>MDSQRNLLVIALLFVSFMIWQAWEQDKNPQPQAQQTTQTTTTAAGSAADQGVPASGQGKLISVKTDVLDLTINTRGGDVEQALLPAYPKELNSTQPFQLLETSPQFIYQAQSGLTGRDGPDNPANGPRPLYNVEKDAYVLAEGQNELQVPMTYTDAAGNTFTKTFVLKRGDYAVNVNYNVQNAGEKPLEISTFGQLKQSITLPPHLDTGSSNFALHTFRGAAYSTPDEKYEKYKFDTIADNENLNISSKGGWVAMLQQYFATAWIPHNDGTNNFYTANLGNGIAAIGYKSQPVLVQPGQTGAMNSTLWVGPEIQDKMAAVAPHLDLTVDYGWLWFISQPLFKLLKWIHSFV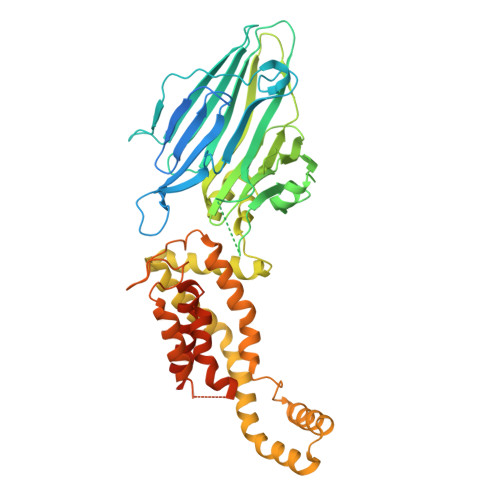GNWGFSIIIITFIVRGIMYPLTKAQYTSMAKMRMLQPKIQAMRERLGDDKQRISQEMMALYKAEKVNPLGGCFPLLIQMPIFLALYYMLMGSVELRQAPFALWIHDLSAQDPYYILPILMGVTMFFIQKMSPTTVTDPMQQKIMTFMPVIFTVFFLWFPSGLVLYYIVSNLVTIIQQQLIYRGLEKRGLLESSGENLYFQ[2x]> MSDVAIVKEGWLHKRGEYIKTWRPRYFLLKNDGTFIGYKERPQDVDQREAPLNNFSVAQCQLMKTERPRPNTFIIRCLQWTTVIEAT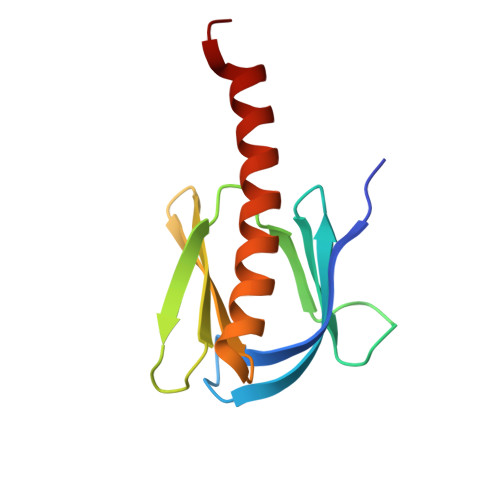FHVETPEEREEWTTAIQTVADGLKKQEEEEMDFR>[4x]AMSDLELRQCLPCGPGGKGRCFGPSI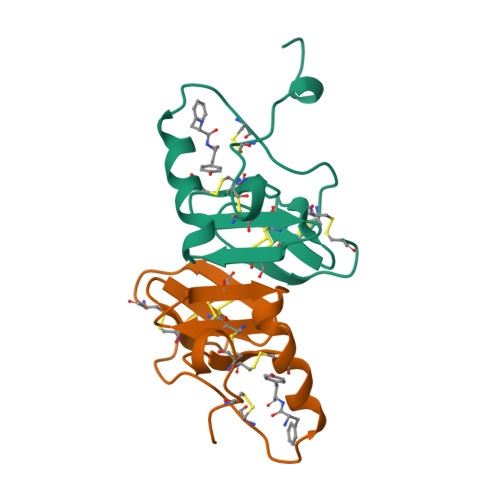CCGDELGCFVGTAEALRCQEENYLPSPCQSGQKPCGSGGRCAAAGICCNDESCVTEPECREGVGFPRRV>MPVAGSELPRRPLPPAAQERDAEPRPPHGELQYLGQIQHILRCGVRKDDRTGTGTLSVFGMQARYSLRDEFPLLTTKRVFWKGVLEELLWFIKGSTNAKELSSKGVKIWDANGSRDFLDSLGFSTR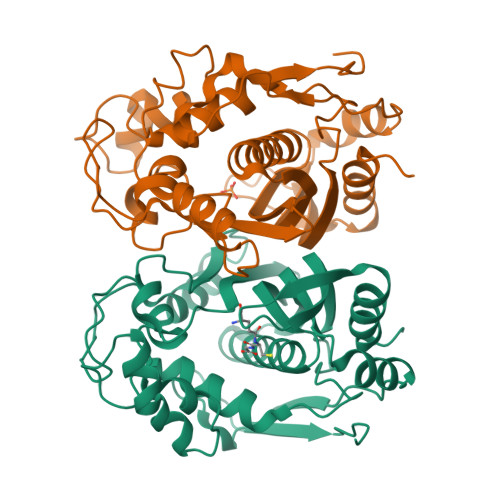EEGDLGPVYGFQWRHFGAEYRDMESDYSGQGVDQLQKVIDTIKTNPDDRRIIMCAWNPRDLPLMALPPCHALCQFYVVNSELSCQLYQRSGDMGLGVPFNIASYALLTYMIAHITGLKPGDFIHTLGDAHIYLNHIEPLKIQLQREPRPFPKLRILRKVEKIDDFKAEDFQIEGYNPHPTIKMEMAV[5x]> GSHHHHHHSQDPMQAAQETKQKLTSCLARRYNAEQKLLDLSALGTDETLSSLGSFNNQSLAEKSFKALMHLVSNEYKDPEQKNEAIQAVSLARNDILDVGQVYSLAVTLPRLRRLDLSGNNLENLSKISKWQQEFRFLEELHLTGNPVTTLPNYATEIKKWFPSLQILDGQQIRTPQEAAESL

The Mex67–Mtr2 complex (NXF1–NXT1 in metazoans and small bristles in Drosophila melanogastor) is the principal mRNA-export factor in Sacccharomyces cerevisiae. Mex67/NXF1 is a modular protein constructed from four domains: an RNA-recognition motif (RRM) domain, a leucine-rich repeat (LRR) domain, a nuclear transport factor 2-like (NTF2L) domain and an ubiquitin-associated (UBA) domain. Mtr2 is a ∼15–20 kDa protein that also has an NTF2-like fold and forms a tight heterodimeric complex with the Mex67 NTF2L domain.

Classically, binding of the RNA cargo has been attributed to the RRM and LRR domains because together these domains are sufficient for Homo sapiens NXF1 to bind the viral RNA CTE (constitutive transport element) sequence motif. d for the ctMex67LRR-NTF2L–Mtr2 (RRM domain deletion) was 6.8 µM, whereas that for ctMex67RRM-LRR (NTF2L–Mtr2 region deletion) was 5.5 µM. These data indicated that as in S. cerevisiae the RRM, LRR and NTF2L–Mtr2 regions all contribute to RNA binding by ctMex67–Mtr2.Here we present rotamer inverted fragment finder–diffusion (Riff-Diff), a hybrid machine learning and atomistic modelling strategy for scaffolding catalytic arrays in de novo proteins. We highlight the general applicability of Riff-Diff by designing enzymes for two mechanistically distinct chemical transformations, the retro-aldol reaction and the Morita–Baylis–Hillman reaction. We show that in both cases, it is possible to generate catalysts that exhibit activities rivalling those optimized by in vitro evolution, along with exquisite stereoselectivity. High-resolution structures of six of the designs revealed near-atomic active site design precision.

We obtained crystal structures of the four designs: RAD13 (kcat = 3.8 × 10−5 s−1), RAD17 (kcat not determined), RAD32 (kcat = 1.1 × 10−2 s−1), and RAD36 (kcat = 6.2 × 10−5 s−1). The crystal structures agree with the design models, having backbone Cα RMSD values between 0.68 Å and 1.2 Å. The catalytic residues of RAD13 and RAD17 adopted the correct conformation with heavy-atom sidechain RMSD values of 0.42 Å and 1.09 Å to the design model and 0.89 Å and 1.2 Å to the catalytic geometry, respectively. Despite the near-atomic precision with which the tetrad was reproduced, RAD13 and RAD17 were more than 105-fold slower than RA95.5-8F. This indicates that precise positioning of catalytic sidechains is by itself not sufficient to design efficient biocatalysts, even when scaffolding catalytic arrays that are derived from highly active enzymes.

> MTPEEEARAAVDSFPEALRQRAWDLNVKSAEKLAKYGIEKVTELALKLLKEIFEKYVEGKITREDLPEVVKKILVLLSLVKATAIYSKEGLEKILELLKEIAKELRERGETLLAEAIDYLIEALEKLHKGDADGYLTLLTIALYLYFKHIVENGARDPELAAAVRPLVEGGYEAVARYYFEVFAPKLEEGTEEAVKLFEE>[4x]GAAEAGITGTWYNQLGSTFIVTAGADGALTGTYESAVGNAESRYVLTGRYDSAPATDGSGTALGWTVAWKNNYRNAHSATTWSGQYVGGAEARINTQWLLTSGTTEANA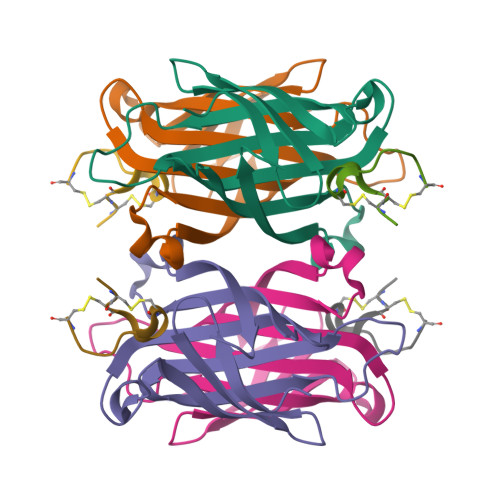WKSTLVGHDTFTKVKPSAAS;>[4x]RCCHPQCGAVEECR MONOIMIDAZOLE 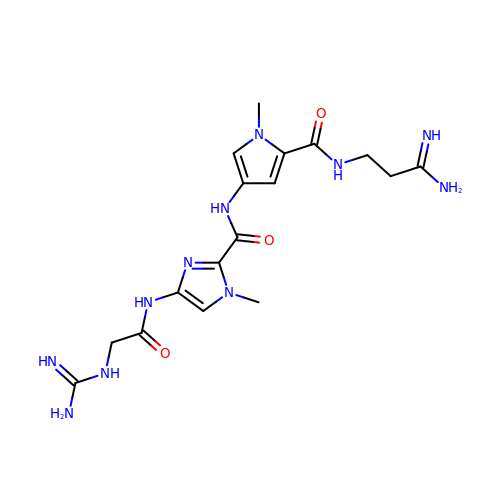LEXITROPSIN | C17 H25 N11 O3 | ZQZPBVXTGJJHBD-UHFFFAOYSA-N>[4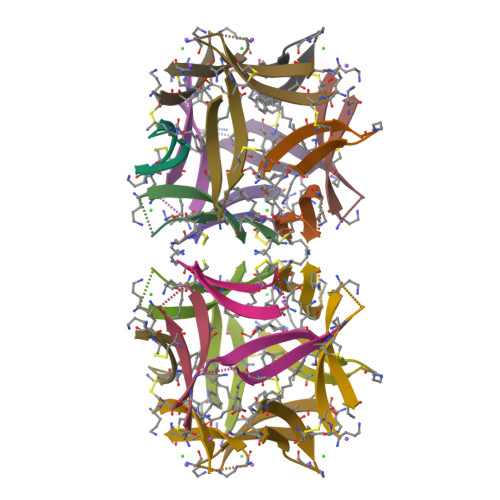x]ACVFFCEDAAIIGLAV> SADAQSFLNRVCGVSAARLTPCGTGTSTDVVYRAFDIYNDKVAGFAKFLKTNCCRFQEKDEDDNLIDSYFVVKRHTFSNYQHEETIYNLLKDCPAVAKHDFFKFRIDGDMVPHISRQRLTKYTMADLVYALRHFDEGNCDTLKEILVTYNCCDDDYFNKKDWYDFVENPDILRVYANLGERVRQALLKTVQFCDAMRNAGIVGVLTLDNQDLNGNWYDFGDFIQTTPGSGVPVVDSYYSLLMPILTLTRALTAESHVDTDLTKPYIKWDLLKYDFTEERLKLFDRYFKYWDQTYHPNCVNCLDDRCILHCANFNVLFSTVFPPTSFGPLVRKIFVDGVPFVVSTGYHFRELGVVHNQDVNLHSSRLSFKELLVYAADPAMHAASGNLLLDKRTTCFSVAALTNNVAFQTVKPGNFNKDFYDFAVSKGFFKEGSSVELKHFFFAQDGNAAISDYDYYRYNLPTMCDIRQLLFVVEVVDKYFDCYDGGCINANQVIVNNLDKSAGFPFNKWGKARLYYDSMSYEDQDALFAYTKRNVIPTITQMNLKYAISAKNRARTVAGVSICSTMTNRQFHQKLLKSIAATRGATVVIGTSKFYGGWHNMLKTVYSDVENPHLMGWDYPKCDRAMPNMLRIMASLVLARKHTTCCSLSHRFYRLANECAQVLSEMVMCGGSLYVKPGGTSSGDATTAYANSVFNICQAVTANVNALLSTDGNKIADKYVRNLQHRLYECLYRNRDVDTDFVNEFYAYLRKHFSMMILSDDAVVCFNSTYASQGLVASIKNFKSVLYYQNNVFMSEAKCWTETDLTKGPHEFCSQHTMLVKQGDDYVYLPYPDPSRILGAGCFVDDIVKTDGTLMIERFVSLAIDAYPLTKHPNQEYADVFHLYLQYIRKLHDELTGHMLDMYSVMLTNDNTSRYWEPEFYEAMYTPHTVLQ;>MAIASEFSSLPSYAAFATAQEAYEQAVANGDSEVVLKKLKKSLNVAKSEFDRDAAMQRKLEKMADQAMTQMYKQARSEDKRAKVTSAMQTMLFTMLRKLDNDALNNIINNARDGCVPLNIIPLTTAAKLMVVIPDYNTYKNTCDGTTFTYASALWEIQQVVDADSKIVQLSEISMDNSPNLAWPLIVTALRANSAVKLQ[2x];> GPVDMSKMSDVKCTSVVLLSVLQQLRVESSSKLWAQCVQLHNDILLAKDTTEAFEKMVSLLSVLLSMQGAVDINKLCEEMLDNRATLQ

The SARS-CoV-2 genome is replicated and transcribed by its RNA-dependent RNA polymerase holoenzyme [holo-RdRp, subunit composition nsp7/nsp82/nsp12 (3, 4)] in a replication–transcription complex (RTC), which is the target for antivirals such as remdesivir (Rdv). The nsp13 helicase translocates on single-stranded nucleic acid in the 5′→3′ direction. Translocation of each enzyme opposes each other, and if the helicase prevails it is expected to push the RdRp backward on the t-RNA. This reversible backward sliding, termed backtracking, is a well-studied feature of the cellular DNA-dependent RNA polymerases (DdRps). Our results establish that the SARS-CoV-2 RTC backtracks, that backtracking is facilitated by the nsp13 helicase, and that the resulting single-stranded 3′ segment of the p-RNA extrudes out the RdRp NTP entry tunnel in a manner analogous to the evolutionarily unrelated cellular DdRps.

The sample comprised two major classes: nsp131-BTC5 (3.4-Å nominal resolution) and nsp132-BTC5 (3.6 Å). To eliminate structural heterogeneity in the nsp13 subunits and obtain a higher-resolution view of the BTC, the particles from both classes were combined and locally refined inside a mask applied around the holo-RdRp and RNA (excluding the nsp13 subunits), leading to the BTC5(local) combined map (3.2 Å). The cryo-EM maps also resolved a single-stranded p-RNA 3′ segment of the BTC5 scaffold extruding into the RdRp NTP entry tunnel, confirming the formation of a BTC. By contrast, the BTC structures were translocated by one base pair compared to the RTCs; the base pair corresponding to the A–U Watson–Crick base pair at the 3′ end of the p-RNA (located in the −1 site of the RTCs) was in the −2 position of the BTCs. The −1 position of the BTC was occupied by the first C–A mismatch; the p-RNA −1C made a non-Watson–Crick hydrogen bond with the opposing t-RNA A. The next three mismatched p-RNA nucleotides (+1C, +2C, and +3C) trailed into the NTP entry tunnel. The 3′ nucleotide of the BTC5 scaffold p-RNA (+4C) was solvent-exposed at the outward-facing end of the NTP entry tunnel and lacked density and was therefore not modeled. The trajectory of the backtracked nucleotides at positions +1/+2 was sharply bent due to spatial constraints of motif F residues. The RdRp NTP entry tunnel provides a steric and electrostatic environment conducive to channeling the backtracked RNA out of the active site without specific polar protein–RNA interactions that could hinder the RNA movement. Our RdRp BTC structures suggest that in the absence of a Mg2+ ion D760 presents an electrostatic barrier to the phosphate backbone of the backtracked RNA, explaining the requirement for the helicase to surmount this barrier and why removal of D760 stabilizes binding to the BTC scaffolds.>[2x]MHHHHHHLVPRGSPARIGYYEIDRTIGKGNFAVVKRATHLVTKAKVAIKIIDKTQLDEENLKKIFREVQIMKMLCHPHIIRLYQVMETERMIYLVTEYASGGEIFDHLVAHGRMAEKEARRKFKQIVTAVYFCHCRNIVHRDLKAENLLLDANLNIKIADFGFSNLFTPGQLLKDWCGSPPYAAPELFEGKEYDGPKVDIWSLGVVLYVLVCGALPFDGST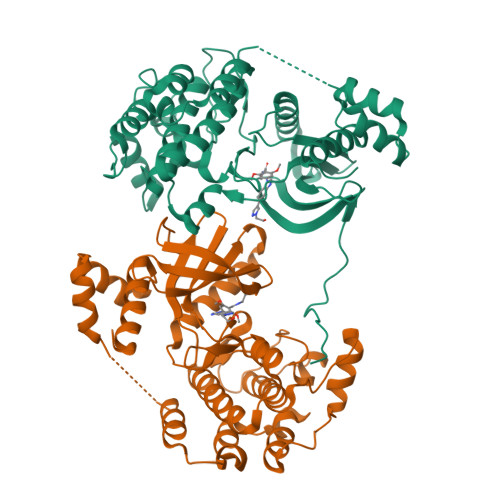LQNLRARVLSGKFRIPFFMSTECEHLIRHMLVLDPNKRLSMEQICKHKWMKLGDADPNFDRLIAECQQLKEERQVDPLNEDVLLAMEDMGLDKEQTLQSLRSDAYDHYSAIYSLLCDRHKRHKTLRL> GMEEDIACVKDLVSKYLADNERLSRQKLAFLVQTEPRMLLMEGLKLLSLCIEIDSCNANGCEHNSEDKSVERILHDHGILTPSLCFVVPDGYKLTGNVLILLECFVRSSPANFEQKYIEDFKKL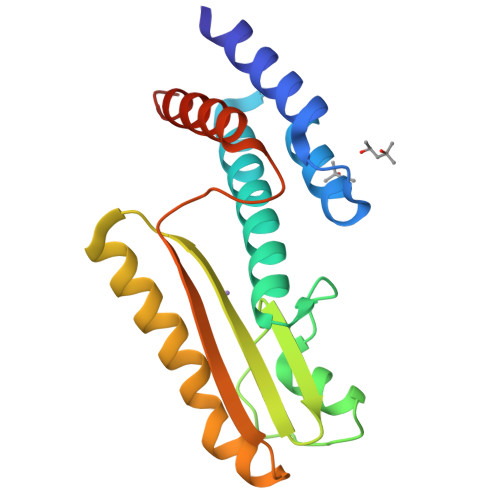EQLKEDLKTVNISLIPLIDGRTSFYNEQIPDWVNDKLRDTLFSLLRYAQES> MPTISVYEDDLFEKLGEEIIEEKLLDVCFDFGLEVDDIEYKNDKKIYKIEVPANRYDLICVEGLCRALKNFMCKFDDIKYDISMNNYDICIKGNQYIKVDGSVDDRRGYVVCCVLKNMNINDSVYNNIIEIQEKLHHNLGKKRSVLAIGIHDYD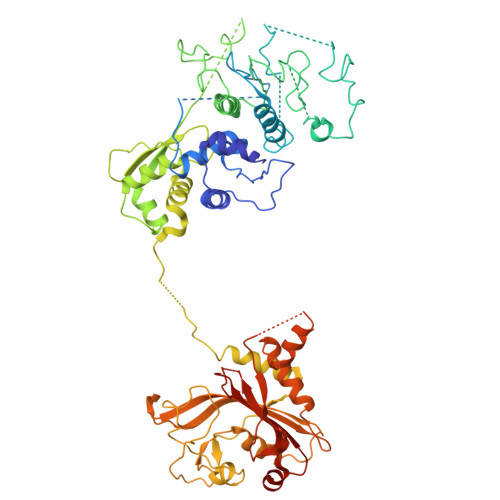KIKFPLKYKFEKKEKINFIPLNEKTNLNGMNLIDFYSKNLNLKPYLKIIKDFDKYPIIVDSNEQILSLPPIINCDHTKISLNTKNVFIECTAIDRNKAQIALNILCSMLSEYCVPKYSIQSFVVIYENQDFSDDQNLKKKETQFLYPIFENKSLTCNIDYVRKLSGISHITVHEVNNLLKRMMLSCDIMDNNTFKVTIPFYRSDIMHCCDIIEDIAIAYGYGNIKYEPPQICKKHSLNNCSELFRNVLVECGYTEVMTNALLSRDENYNCMLRTHKSYDDPNINLDEYNPLAAPIQIKNSKTSEYEIIRTSLIVNLLKFVSANKHRELPLRFFEIGDVSYATYNQTDTNAVNKKYLSIIFSDKFTAGLEELHGVLEAILKEYQLFSDYKIEEKKKENISIRSDMYYKLIPKEDPSFLNERIVDIVLFPHNLKFGVLGIIHPKVLENFSLDIPVSAIEINVETLLNVLMM> SLQRVPSYDSFDSEDYPAALPNHKPKGTFKDYVRDRADLNKDKPVIPAAALAGYTGSPPIQLWQFLLELLTDKSCQSFISWTGDGWEFKLSDPDEVARRWGKRKNKPKMNYEKLSRGLRYYYDKNIIHKTAGKRYVYRFVCD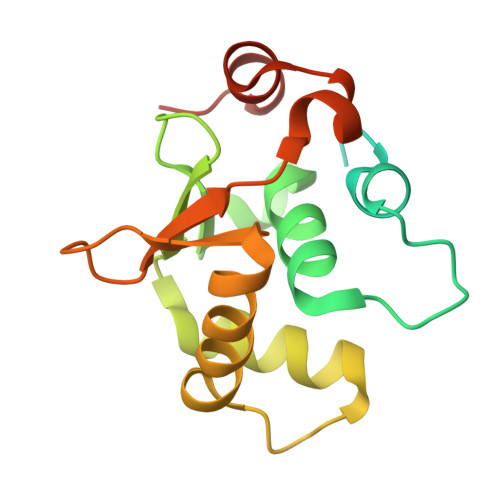LQSLLGYTPEELHAMLDVKPDADE> KSDVTAQDVENALTDTSKNVELTVWAYSAKQMEPTVKAFEKKY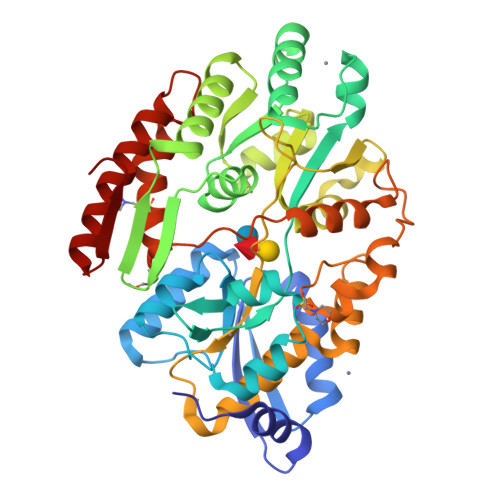PHIKINFVNTGAAEDHFTKFQNVVQAQKDIPDVVQMSANKFQQFAVSGALLNFANDSIEKAWSKLYTKTAWAQVHYAGGLYGAPQDATPLANYVRKDILDEHNLQVPESWEDIYNEGIKLHKEDSNKYMGILGSDISFFTNLYRSVGARLWKVNSVDDVELTMNSGKAKEFTEFLQKCLKDGVLEGGTVFTDEFNRSINDGRYATFINENWMGNTYKEQNPSLKGKMVVAAPPSWKGQPYQSSSVGSMMSVSAACPKEKQAAALAFINWLDSDKDAIQSWQDTNNGNFFMAASVYQDDENQRNKKETDGYYANDDVNAVYFDSMDKVNTDWEYLPFMSQVEVVFNDVIVPEMNENGDLVGAMAKAQQKLKAYAEDNGFKVTTDAD> MPQSKSRKIAILGYRSVGKSSLTIQFVEGQFVDSYDPTIENTFTKLITVNGQEYHLQLVDTAGQDEYSIFPQTYSIDINGYILVYSVTSIKSFEVIKVIHGKLLDMVGKVQIPIMLVGNKKDLHMERVISYEEGKALAESWNAAFLESSAKENQTAVDVFRRIILEAEKMDGACSQG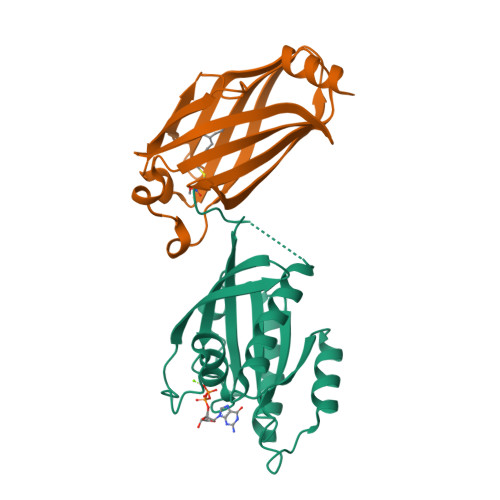KSSC;> GSMSAKDERAREILRGFKLNWMNLRDAETGKILWQGTEDLSVPGVEHEARVPKKILKCKAVSRELNFSSTEQMEKFRLEQKVYFKGQCLEEWFFEFGFVIPNSTNTWQSLIEAAPESQMMPASVLTGNVIIETKFFDDDLLVSTSRVRLFYV>TAGGGTTAGGGTTAGGGTT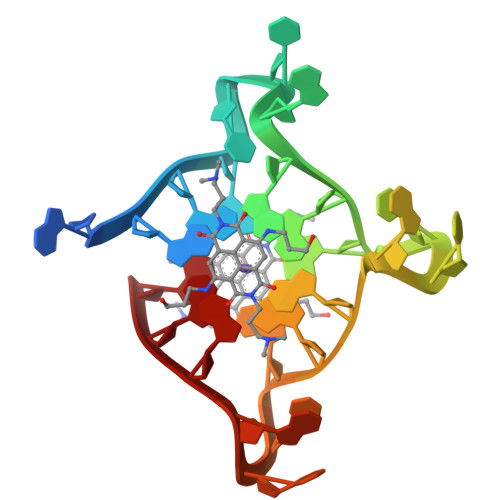AGGG[2x]>MNENEKKLTTNQGVPIGDNQNSRTAGRRGPTLLEDYQLIEKIAHFDRERVPERVVHARGFGAHGVFKVKNSMKKYTKAAFLQEEGTEVPVFARFSTVIHGTHSPETLRDPRGFSVKFYTEEGNWDFVGNNLPVFFIRDAMKFPDMVHSLKPDPRTNIQDPDRYWDFMTLRPESTNMLMHIFTDEGIPASYRKMRGSSVHSFKWVNAHGNTVYIKLRWVPKEGVHNLSADEATEVQGKDFNHASNDTFQAIENGDFPEWDLFVQVLDPADVENFDFDPLDATKDWFEDVIPFQHVGTMTLNKNVDNYFAETESVGFNPGVLVPGMLPSEDKLLQGRLFSYSDTQRHRIGPNYQQLPINCPFAQVNNYQRDGAMPFKQQTSSVNYEPNRYQDEPKQTPEYTEDTQPLHDDIHGRLEIEKTNNFGQAGEVYRRM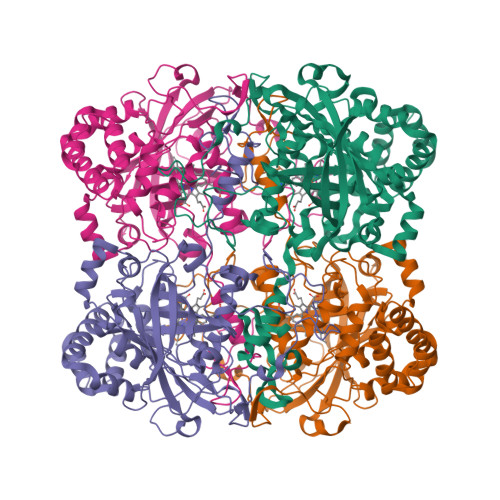TEEEQMALLNNLVNDLQQVRHENTVLLAICNFYRADASLGEKLSEALNVDIKPFLQQMQK[4x]> MGSSHHHHHHSQDPGDENLYFQSMSTEVETEKPAPVAYPFTGSEGLELSQSYAKLFEDGDPIRVQLPFGEPAWLVTRYDDARFVLTDRRFSRHLATQRDEPRMTPRAVPESILTMDPPDHTRLRTLVSKAFTPRRIESKRAWIGELAAGLVADMKAGGAPAELVGSYALAIPVTVICELLGVPEDDRTRLRGWCDAALSTGELTDEECVQSFMDLQKYFEDLVKERRAEPRDDLTSALIEARDAHDRLAEPELIGLCISILIGGFETTASEISSFVHVL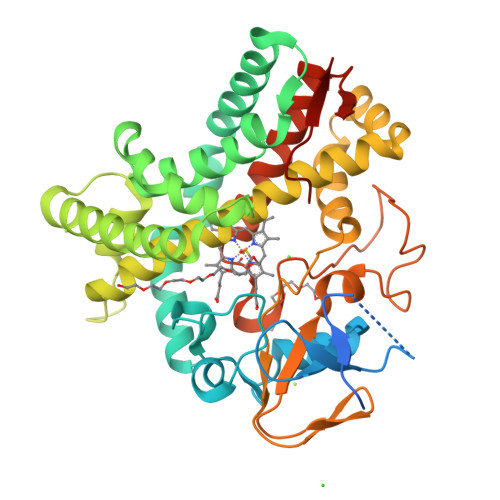QQRRELWTRLCADPEAIPAAVEELLRFVPFAANGISPRYALEDMTVGGVLVREGEPVIVDTSAVNRDGLVFDNADEVVIDRADNRHMVFGHGAHHCLGAHLARVELQEALKALVEGMPGLRLSGDVEWKADMIIRAPRVMHVEW>GMLSLELCDDDPPEIPHATFKAMAYKEGTMLNCECKRGFRRIKSGSLYMLCTGSSSHSSWDNQCQCTSSATRSTTKQVTPQPEEQKERKTTEMQSPMQPVDQASLPGHCREPPPWENEATERIYHFVVGQMVYYQCVQGYRALHRGPAESVCKMTHGKTRWTQPQLICTGEMETSQFPGEEKPQASPEGRPESETSCLVTTTDFQIQTEMAATMETSTGHHHHHH[2x];>[2x]GMLSLAVNGTSQFTCFYNSRANISCVWSQDGALQDTSCQVHAWPDRRRWNQTCELLPVSQASWACNLILGAPDSQKLTTVDIVTLRVLCREGVRWRVMAIQDFKPFENLRLMAPISLQVVHVETHRCNISWEISQASHYFERHLEFEARTLSPGHTWEEAPLLTLKQKQEWICLETLTPDTQYEFQVRVKPLQGEFTTWSPWSQPLAFRTKTGHHHHHH;>GMLSLLNTTILTPNGNEDTTADFFLTTMPTDSLSVSTLPLPEVQCFVFNVEYMNCTWQSSSEPQPTNLTLHYWYKNSDNDKVQKCSHYLFSEEITSGCQLQKKEIHLYQTFVVQLQDPREPRRQATQMLKLQNLVIPWAPENLTLHKLSESQLELNWNNRFLNHCLEHLVQYRTDWDHSWTEQSVDYRHKFSLPSVDGQKRYTFRVRSRFNPLCGSAQHWSEWSHPIHWGSNTSKENPRTGHHHHHH[2x];>APTSSSTKKTQLQLEHLLLDLQMILNGINNYKNPKLTRMLTFKFYMPKKATELKHLQCLEEELKPLEEVLNLAQSKNFHLRPRDLISNINV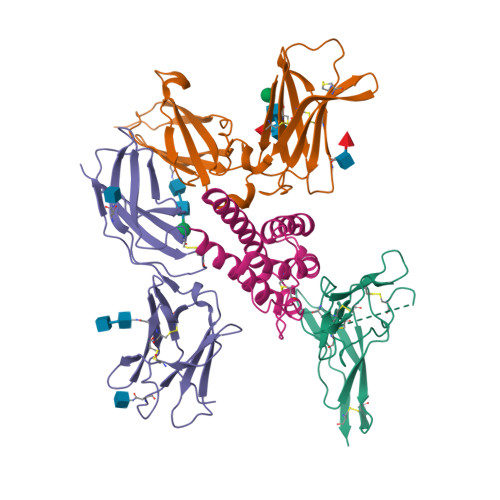IVLELKGSETTFMCEYADETATIVEFLNRWITFAQSIISTLT[2x]> MHHHHHHHPGFFTSIGQMTDLIHTEKDLVTSLKDYIKAEEDKLEQIKKWAEKLDRLTSTATKDPEGFVGHPVNAFKLMKRLNTEWSELENLVLKDMSDGFISNLTIQRQYFPNDEDQVGAAKALLRLQDTYNLDTDTISKGNLPGVKHKSFLTAEDCFELGKVAYTEADYYHT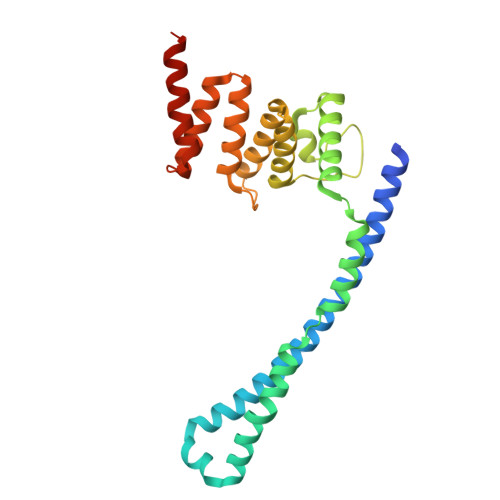ELWMEQALRQLDEGEISTIDKVSVLDYLSYAVYQQGDLDKALLLTKKLLELDPEHQRANGNLKYFEYIMAKEKDVNKS> MKTQVAIIGAGPSGLLLGQLLHKAGIDNVILERQTPDYVLGRIRAGVLEQGMVDLLREAGVDRRMARDGLVHEGVEIAFAGQRRRIDLKRLSGGKTVTVYGQTEVTRDLMEAREAC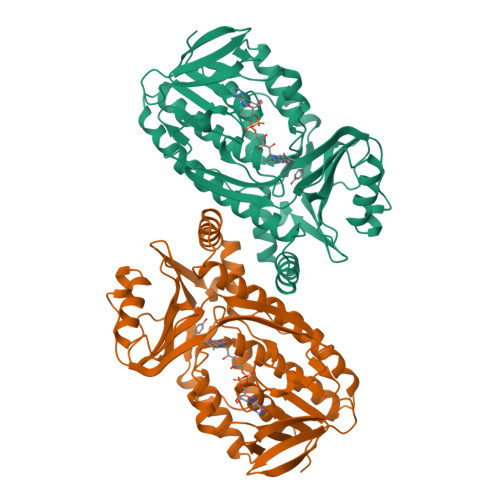GATTVYQAAEVRLHDLQGERPYVTFERDGERLRLDCDYIAGCDGFHGISRQSIPAERLKVFERVYPFGWLGLLADTPPVSHELIYANHPRGFALCSQRSATRSRYYVQVPLSEKVEDWSDERFWTELKARLPSEVAEKLVTGPSLEKSIAPLRSFVVEPMQHGRLFLAGDAAHIVPPTGAKGLNLAASDVSTLYRLLLKAYREGRGELLERYSAICLRRIWKAERFSWWMTSVLHRFPDTDAFSQRIQQTELEYYLGSEAGLATIAENFVGLPYEEIE(3~{S})-3-azanyl-4-(4-bromophenyl)-~{N}-[(3~{S})-1-[2-[[(2~{R})-1-(3,4-dichlorophenyl)-4-(methylamino)-4-oxidanylidene-butan-2-yl]amino]-2-oxidanylidene-ethyl]-2-oxidanylidene-4,5-dihydro-3~{H}-1-benzazepin-3-yl]butanamide 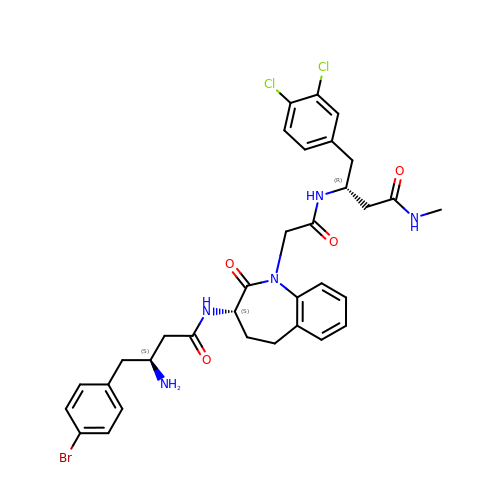| C33 H36 Br Cl2 N5 O4 | CCMSKSUYUVJSCD-OARDWFSCSA-N> MGHHHHHHDSPVLMVYGLDQSKMNCDRV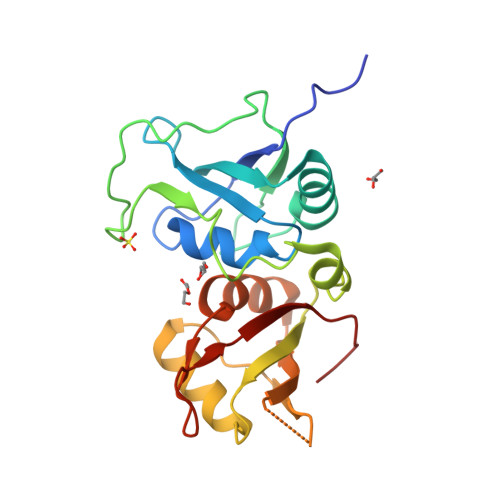FNVFCLYGNVEKVKFMKSKPGAAMVEMADGYAVDRAITHLNNNFMFGQKLNVCVSKQPAIMPGQSYGLEDGSCSYKDFSESRNNRFSTPEQAAKNRIQHPSNVLHFFNAPLEVTEENFFEICDELGVKRPSSVKVFSGKSERSSSGLLEWESKSDALETLGFLNHYQMKNPNGPYPYTLKLCFSTAQHAS> MASPDEDNPGILYNGRFDFSDPNGPKCAWSGSNVELNFYGTEASVTIKSGGENWFQAIVDGNPLPPFSVNATTSTVKLVSGLAEGAHHLVLWKRTEASLGEVQFLGFDFGSGKLLAAPKPLERKIEFIGDAITCAYGNEGTSKEQSFTPKNENSYMSYAAITARNLNASANMIAWSGIGLTMNYGGAPGPLIMDRYPYTLPYSGVRWDFSKYVPQVVVINLGT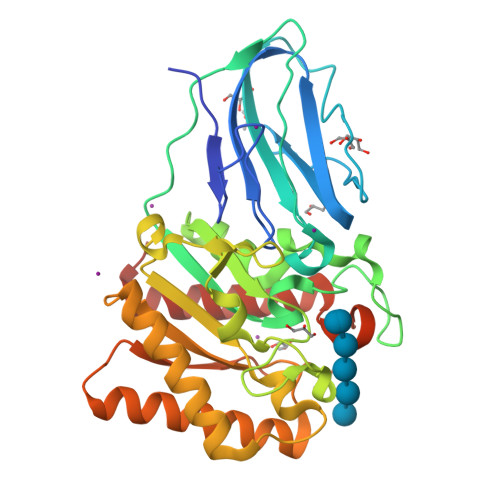NDFSTSFADKTKFVTAYKNLISEVRRNYPDAHIFCCVGPMLWGTGLDLCRSYVTEVVNDCNRSGDLKVYFVEFPQQDGSTGYGEDWHPSIATHQLMAERLTAEIKNKLGWLEHHHHHH>[10x]MSCGAAKLNHPAPEFDDMALMPNGTFKKVSLSSYKGKYVVLFFYPMDFTFVCPTEIIQFSDDAKRFAEINTEVISCSCDSEYSHLQWTSVDRKKGGLGPMAIPMLAD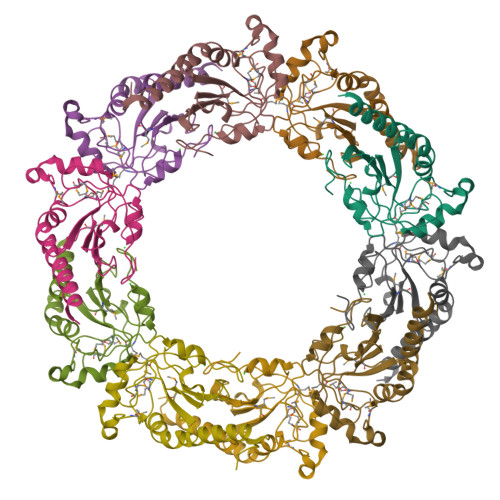KTKAIARAYGVLDEDSGVAYRGVFIIDPNGKLRQIIINDMPIGRNVEEVIRLVEALQFVEEHGEVCPANWKKGDAKKKEGH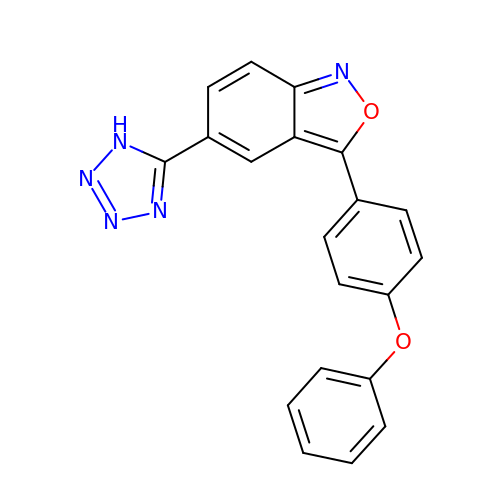(5P)-3-(4-phenoxyphenyl)-5-(1H-tetrazol-5-yl)-2,1-benzoxazole | C20 H13 N5 O2 | RMVHXXZAXAMVLU-UHFFFAOYSA-N> MFTNTIERVNFASAKNIPEYPDFLDIQIKSFQDFFQLETKSDERGNEGLYNTFMENFPITDTRNQFVLEFLDYFIDPPRYSIQECIERGLTYSVPLKARLKLYCTDPEHEDFETIVQDVYLGTIPYMTPSGTFVINGAERVVVSQLHRSPGVFFGQSFHANGTKLYSARVIPFKGSWIEFATDINGVMYAYIDRKKKLPVTTLFRAIGFERDKDILEIFDLSEEVKVSKAGLKKVLGRKLAARVLNTWHEDFVDEDTGEVVSIERNEIILDRDTILEKEHIDEIIDADVKTILLHKENNAQSDYAIIHNTLQKDPTNSEKEAVEHIYRQLRNAEPPDEETARGIIEKLFFSDQRYSLGEVGRYRMNKKLGLDIGMDKEVLTKEDIITIIKYLIELINSKAEIDDIDHLSNRRVRTVGEQLSQQFGVGLARMARTIRERMNVRDNEVFTPIDLINAKTLSSVINSFFGTNQLSQFMDQTNPLAEITHKRRLSALGPGGLSRERAGFEVRDVHYTHYGRLCPIETPEGPNIGLISSLSVFAKVNSMGFLETPYRKVVDGKVDVKEHIYLSAEEEEGMKIAQANIPLKDDGTIDREKVIARDEGDFPVVDPVEINYTDVAPNQIASISASLIPFLEHDDANRALMGSNMMRQAVPLLRPESPIVGTGLERQVATDSRVLINAEGDGVVEYVDAQKITIKYDRTEEERLVSFEEDSKTYELVKFRKTNQGTSINLKPIVRKGDKVKKGQVLCEGYATEKGELALGRNMKVAFMPWKGYNFEDAIVISEKVVREDIFTSVHIDEYALEVRDTKLGAEELTNDIPNVSEEATRDLDEYGMIRIGAEVKPGDILIGKITPKGESDPTPEEKLLRAIFGDKAGDVKDASLKASPSLRGVVIDKKLFSRSIKDKRKRSEDKEAISRLEMDYEVKFQQLKDVLIEKLFGLVNGKTSQGVINDLGEEVLPKGKKYTIKMLNAVDDFAHLVGGSWTTDEDTNALVADLLHNYKIKLNDIQGNLRRDKFTISVGDELPAGIMKLAKVYIAKKRKLKVGDKMAGRHGNKGIVARIVRQEDMPFLEDGTPVDIVLNPLGVPSRMNIGQIYETVLGWAGLKLGQKYGTPIFDGATLDDINELTDKAGVPRFGHTYLYDGGTGQRFDQAATVGVIYMLKLGHMVDDKMHARSIGPYSLITQQPLG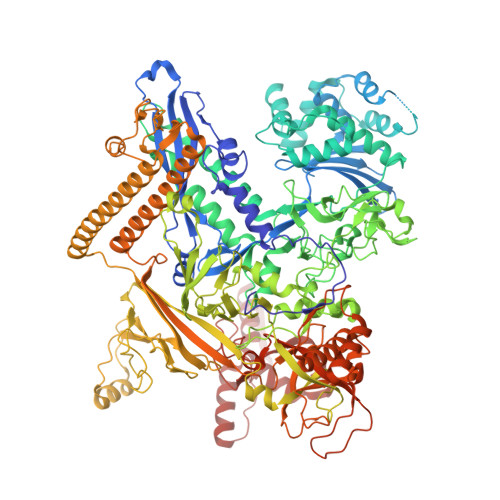GKAQFGGQRFGEMEVWALEAYGASATLREILTVKSDDVIGRAKTYESIVKGETMPEPGLPESFNVLMHELKGLGLDIRLEE>MGSDKIHHHHHHMKIDILDKGFVELVDVMGNDLSAVRAARVSFDMGLKDEERDRHLIEYLMKHGHETPFEHIVFTFHVKAPIFVARQWFRHRIASYNELSGRFSKLSYEFYIPSPERLEGYKTTIPPERVTEKISEIVDKAYRTYLELIESGVPREVARIVLPLNLYTRFFWTVNARSLMNFLNLRADSHAQWEIQQYALAIARIFKEKCPWTFEAFLKYAYKGDILKEVQV[4x]

Many microbes, including human pathogens, utilize the flavin-dependent thymidylate synthase encoded by the thyX gene to generate dTMP. The mechanism of action relies on the reduced coenzyme FADH−, which acts both as a mediator, facilitating methylene transfer from CH2THF to dUMP, and as a reducing agent. As expected, the enzyme formed a tetramer where four identical active sites forming large cavities were generated at the interface of three different monomers. Here, we report the crystal structures of T. maritima ThyXred alone and in the presence of dUMP as well as the crystal structures of the ThyX Y91F mutant with FAD in the oxidized and reduced form.

As mentioned, the interaction between Y91 and H53 could be a key factor in the closed conformation of the folate site. To investigate this further, we generated the Y91F ThyX mutant and characterized it. The Y91F mutant has a flavin content similar to that of the WT, but with different absorption spectra of the reduced forms, indicating an altered flavin environment in the mutant. In addition, mutation of this Y91 has been shown to induce a 1000-fold decrease in flavin oxidation rate during the methylation reaction compared with the WT.> MERNKLARQIIDTCLEMTRLGLNQGTGNVSVRYQDGMLITPTGIPYEKLTESHIVFIDGNGKHEEGKLPSSEWRFHMAAYQSRPDANAVVHNHAVHCTAVSILNRSIPAIHYMIAAAGGNSIPCAPYATFGTRELSEHVALALKNRKATLLQHHGLIACEVNLEKALWLAHEVEVLAQLYLTTLAI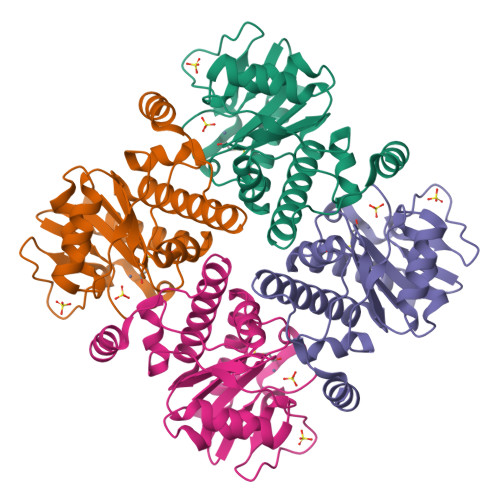TDPVPVLSDEEIAVVLEKFKTFGLRIEE> MQVFIMRHGDAALDAASDSVRPLTTNGCDESRLMANWLKGQ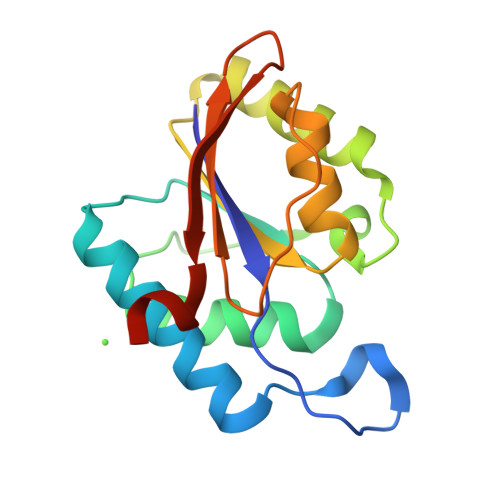KVEIERVLVSPFLRAEQTLEEVGDCLNLPSSAEVLPELTPCGDVGLVSAYLQALTNEGVASVLVISHLPLVGYLVAELCPGETPPMFTTSAIASVTLDESGNGTFNWQMSPCNLKMAKAI> MLRVDQTGTILIKNGTVVNDDRYFKSDVLVENGIIKEISKNIEPKEGIKVVDATDKLLLPGGIDTHTHFQLPFMGTVSVDDFDIGTQAAVAGGTTFIIDFVIPTRGQSLLEAYDQWKKWADEKVNCDYSLHVAITWWSEQVSREMEILVKERGVNSFKCFMAYKNSFMVTDQEMYHIFKRCKELGAIAQVHAENGDMVFEGQKKMLEMGITGPEGHELSRPEALEAEATNRAIVIADSVCTPVYIVHVQSIGAADVICKHRKEGVRVYGEPIAAGLGVDGSHMWNHDWRHAAAFVMGPPIRPDPRTKGVLMDYLARGDLDCVGTDNCTFCADQKAMGKDDFTKIPNGVNGVEDRMSIVWENGVNTGKLTWCQFVRATSSERARIFNIYPRKGRIDVGCDGDIVIWDPNQSKTISKDTHHHAVDFNIFEGIKVTGIAVTTIVAGNIVWSDNKLSCV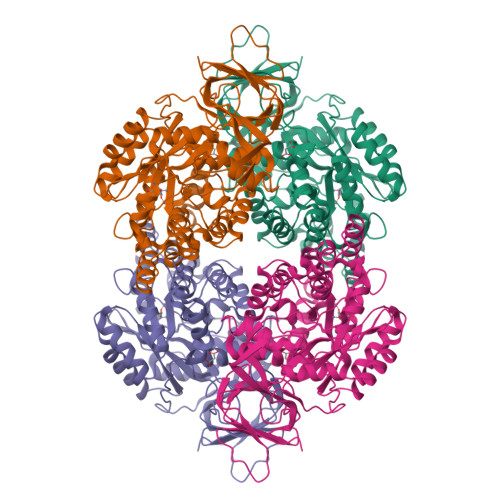KGSGRFVPRPPFGPVFDGIEQRDKVRNELLRKVDRKPYEDDNTKNSSKPGDDDDKHHHHHHHHSGD> VTGEEVLQNACAACHVQHEDGRWERIDAARKTPEGWDMTVTRMMRNHGVALEPEERAAIVRHLSDTRGLSLAETEERRYILEREPVAWDEGPDTSMTQTCGRCHSYARVALQRRTPEDWKHLVNFHLGQFPTLEYQALARDRDWWGIAQAEIIPFLARTYPLGEAPDAYADDASGAYVLAGRQPGRGDYTGRLVLKKAGEDYEVTMTLDFADGSRSFSGTGRILGAGEWRATLSDGTVTIRQIFALQDGRFSGRWHDADSDVIGGRLAAVKADAAPQVLAVAPARLKIGEETQLRVAGTGLGSDLTLPEGVAGSVESAGNGVTVLKLTATGTP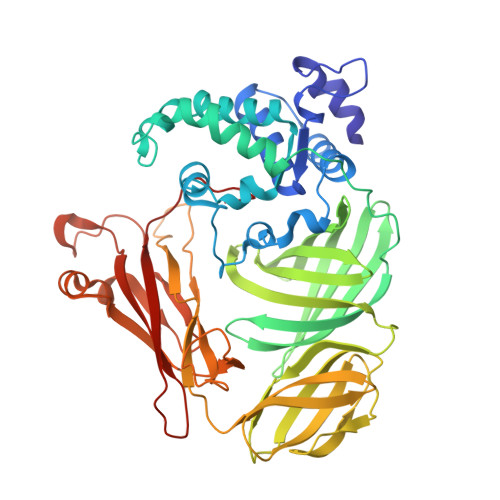GPVSLELGGQKVDLVAYDRPDRISIVPDLTIARIGGNGGPIPKVPAQFEAMGWLNGPDGQPGTGDDIALGAFPASWATDNFDEEAEKMQDAKYAGSIDDTGLFTPAEAGPNPERPMQTNNAGNLKVIATVDAEGEPLSAEAHLYATVQRFVDAPIR> GSHMTDLPRLPFDNPDIMGIAPQMLALQKEGPIARVGTAGEDAWLVTRYDEVRTLLADRRLRLSNPNPQPSAKSAARAFMVALMAGDDHETEPARHAQMRSLLIPRFSTRRLRLMKTRIEHHVDELLDQLAASAPPVDLHRVLSFRLPTMVVCDLLGVPLADRERFGQWARGTFDQSDNEHSANTFQQVVDYMLELVARKRVEPGDDILSELIAEKDGALSDADIAHLGNAVLLLGYETTIVRIDLGTLLLLRNPVQRAQLAEDPGLAPAAVEEILRLGVGGKGSNALIPRYAHGDITVGETVIRTGDAVMLAIGAANYDDRAFPDGG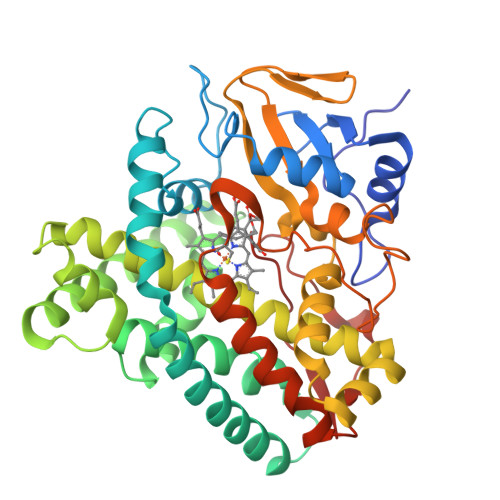LFDLTRVRPRSHLAFGHGARHCIGRTLARIELTAVFERLFRRLPDLRLAVPEESLRWQEHRITGGFDEIPVTF> GVQLTAAQELMIQQLVAAQLQCNKRSFSDQPKVTPWPLGADPQSRDARQQRFAHFTELAIISVQEIVDFAKQVPGFLQLGREDQI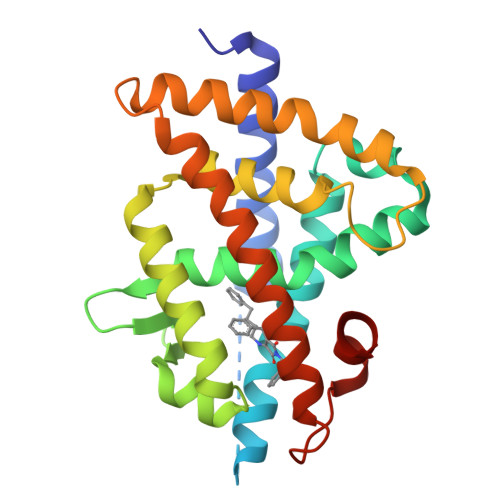ALLKASTIEIMLLETARRYNHETECITFLKDFTYSKDDFHRAGLQVEFINPIFEFSRAMRRLGLDDAEYALLIAINIFSADRPNVQEPGRVEALQQPYVEALLSYTRIKRPQDQLRFPRMLMKLVSLRTLSSVHSEQVFALRLQDKKLPPLLSEIWDVHE>MEFRQLKYFIAVAEAGNMAAAAKRLHVSQPPITRQMQALEADLGVVLLERSHRGIELTA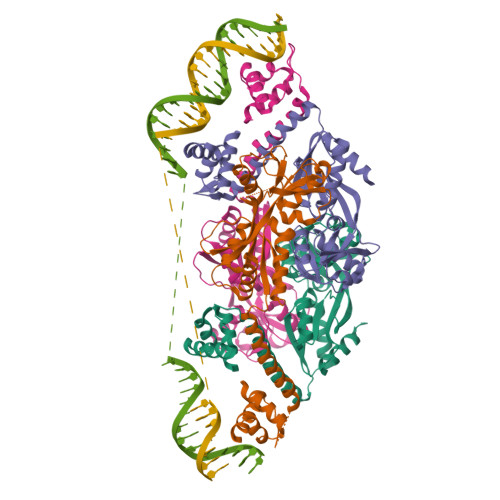AGHAFLEDARRILELAGRSGDRSRAAARGDVGELSVAYFGTPIYRSLPLLLRAFLTSTPTATVSLTHMTKDEQVEGLLAGTIHVGFSRFFPRHPGIEIVNIAQEDLYLAVHRSQSGKFGKTCKLADLRAVELTLFPRGGRPSFADEVIGLFKHAGIEPRIARVVEDATAALALTMAGAASSIVPASVAAIRWPDIAFARIVGTRVKVPISCIFRKEKQPPILARFVEHVRRSAKD[4x]> MHRTTRIKITELNPHLMCVLCGGYFIDATTIIECLHSFCKTCIVRYLETSKYCPICDVQVHKTRPLLNIRSDKTLQDIVYKLVPGLFKNEMKRRRDFYAAHPSADAAN;> GPLGSHMSQAVQTNGTQPLSKTW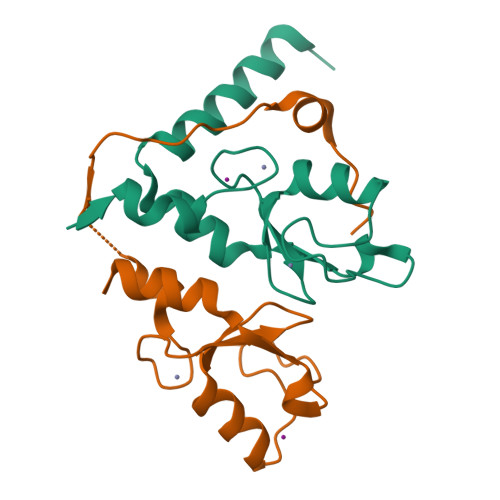ELSLYELQRTPQEAITDGLEIVVSPRSLHSELMCPICLDMLKNTMTTKECLHRFCADCIITALRSGNKECPTCRKKLVSKRSLRPDPNFDALISKIYPSRDEYEAHQERVLARINKHNNQQALSHSIEEGLKIQAMNRLQRG>[2x]GSHMGQGGSNPKFENIAEGLRALLARSHVERTTDEGTWVAGVFVYGGSKTSLYNLRRGTALAIPQCRLTPLSRLPFGMAPGPGPQPGPLRESIVCYFMV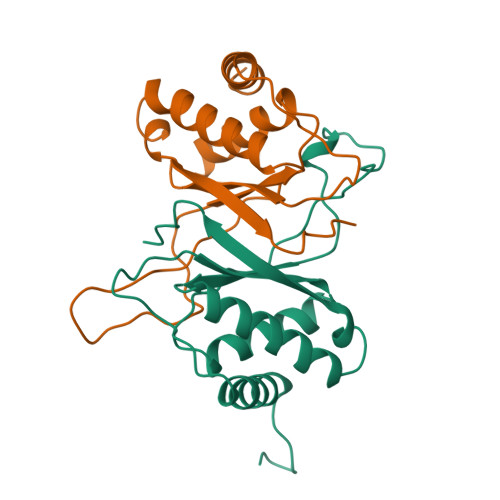FLQTHIFAEVLKDAIKDLVMTKPAPTCNIRVTVCSFDDGVDLP>[2x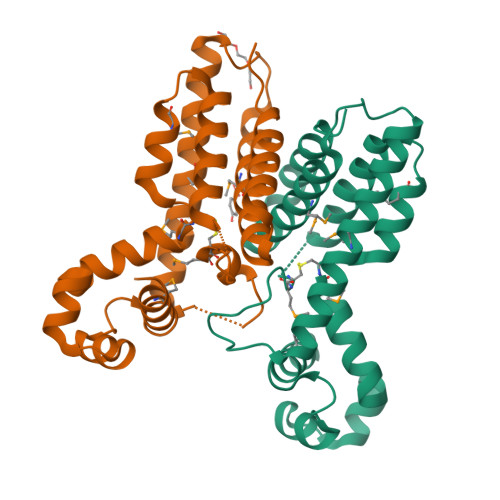]GHMPGGRRRGFDDQVALQTAMELFWRQGYEGTSITDLTKALGINPPSLYAAFGSKRDLFEKTLDRYMCERTLQLEEAMVRPTAHEAVLDFLTGRVEVFTAPGQPFGCMTVQAGLASGEPHHEIVDLLTAAREQMRQTVLDRFEKALADGDLPAGTDCTALARYVMAAVYGLSVEAASGAPREELTAAAILAAQVVPRAQMGS>[4x]NLSDDLSFNFDKFVPNQKNIIFQGDASVSTTGVLQVTKVSKPTTTSIGRALYAAPIQIWDSITGKVA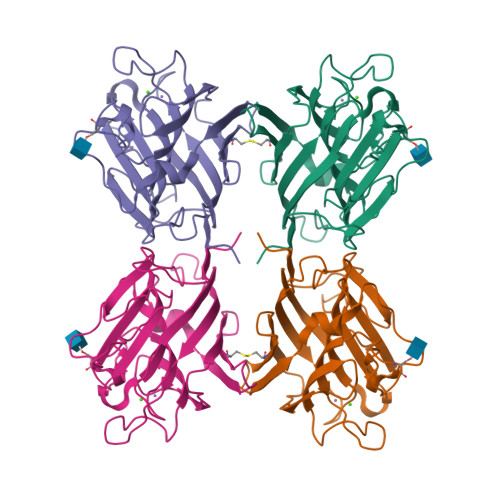SFATSFSFVVKADKSDGVDGLAFFLAPANSQIPSGSSAGMFGLFSSSDSKSSNQIIAVEFDTYFGKAYNPWDPDFKHIGIDVNSIKSIKTVKWDWRNGEVADVVITYRAPTKSLTVCLSYPSDGTSNIITASVDLKAILPEWVSVGFSGGVGNAAEFETHDVLSWYFTSNLEANN> MGSSHHHHHHSQDPNSNQAQELNHELELEQLETKITVSSVSLTGS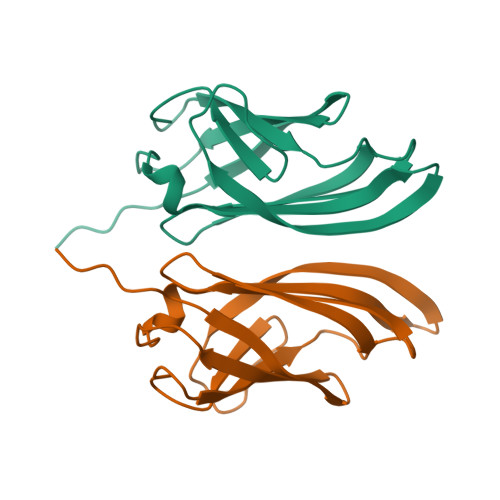TLNVVLENNGSTNLYDFQGFSVIVQYYANISNISTFNLSLYNYTKNSNPSPYYWTINTPLLAPGSQATLTIILPYPPYPNTQATVVIVTNYGPSVIWRGSL>GGGGTTTTGG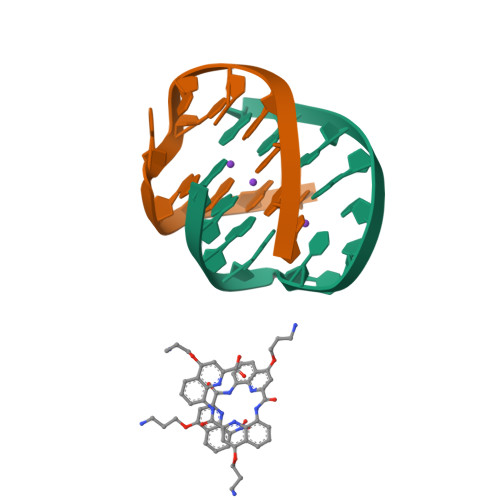GG[2x]>[4x]GPLGSRLFSRFD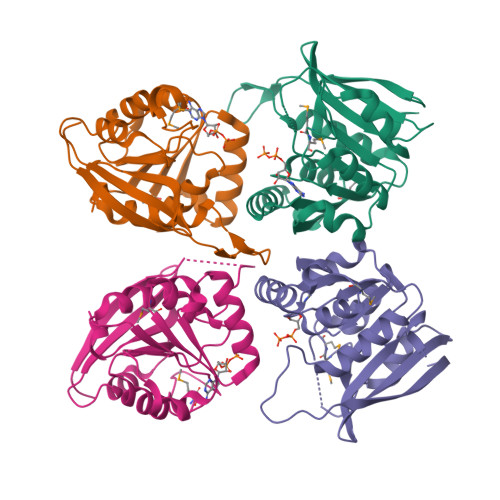DGIKLDREGWFSVTPEKIAEHIAGRVSQSFKCDVVVDAFCGVGGNTIQFALTGMRVIAIDIDPVKIALARNNAEVYGIADKIEFICGDFLLLASFLKADVVFLSPPWGGPDYATAETFDIRTMMSPDGFEIFRLSKKITNNIVYFLPRNADIDQVASLAGPGGQVEIEQNFLNNKLKTITAYFGDLIRRPASET[2-(phenylamino)benzene-1,4-diyl]bis{[4-(pyrrolidin-1-yl)piperidin-1-yl]methanone} 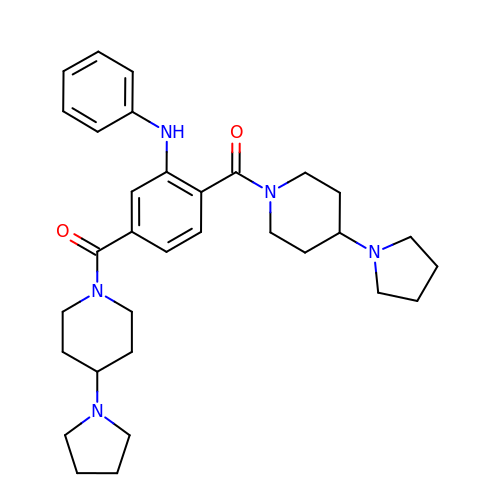| C32 H43 N5 O2 | PQOOIERVZAXHBP-UHFFFAOYSA-N> MFDKILIANRGEIACRIIKTAQKMGIKTVAVYSDADRDAVHVAMADEAVHIGPAPAAQSYLLIEKIIDACKQTGAQAVHPGYGFLSERESFPKALAEAGIVFIGPNPGAIAAMGDKIESKKAAAAAEVSTVPGFLGVIESPEHAVTIADEIGYPVMIKASAGGGGKGMRIAESADEVAEGFARAKSEASSSFGDDRVFVEKFITDP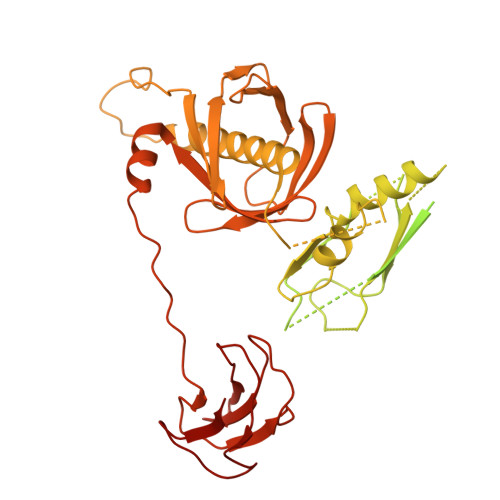RHIEIQVIGDKHGNVIYLGERECSIQRRNQKVIEEAPSPLLDEETRRKMGEQAVALAKAVNYDSAGTVEFVAGQDKSFYFLEMNTRLQVEHPVTEMITGLDLVELMIRVAAGEKLPLSQDQVKLDGWAVESRVYAEDPTRNFLPSIGRLTTYQPPEEGPLGGAIVRNDTGVEEGGEIAIHYDPMIAKLVTWAPTRLEAIEAQATALDAFAIEGIRHNIPFLATLMAHPRWRDGRLSTGFIKEEFPEGFIAPEPEGPVAHRLAAVAAAIDHKLNIRKRGISGQMRDPSLLTFQRERVVVLSGQRFNVTVDPDGDDLLVTFDDGTTAPVRSAWRPGAPVWSGTVGDQSVAIQVRPLLNGVFLQHAGAAAEARVFTRREAELADLMPVKENAGSGKQLLCPMPGLVKQIMVSEGQEVKNGEPLAIVEAMKMENVLRAERDGTISKIAAKEGDSLAVDAVILEFA> GHMSVAAGDKPTNSRQEILEGARRCFAEHGYEGATVRRLEEATGKSRGAIFHHFGDKENLFLALAREDAARMAEVVSENGLVEVMRGMLEDPERYDWMSVRLEISKQLRTDPVFRAKWIDHQSVLDEAVRVRLSRNVDKGQMRTDVPIEVL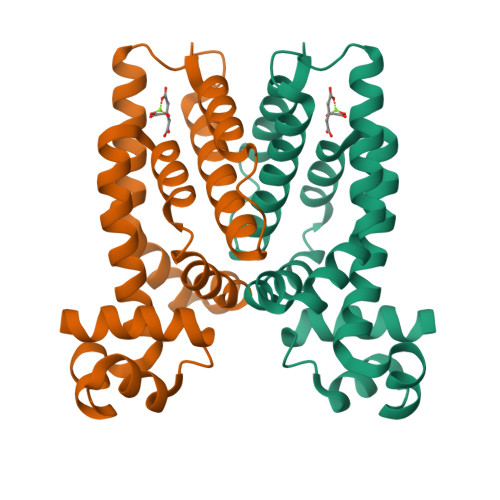HTFLETVLDGFISRLATGASTEGLSEVLDLVEGTVRKRD> MNITKPFPLPTGYFGIPLGLAALSLAWFHLENLFPAARMVSDVLGIVASAVWILFILMYAYKLRYYFEEVRAEYHSPVRFSFIALIPITTMLVGDILYRWNPLIAEVLIWIGTIGQLLFSTLRVSELWQGGVFEQKSTHPSFYLPAVAANFTSASSLALLGYHDLGYLFFGAGMIAWIIFEPVLLQHLRISSLEPQFRATMGIVLAP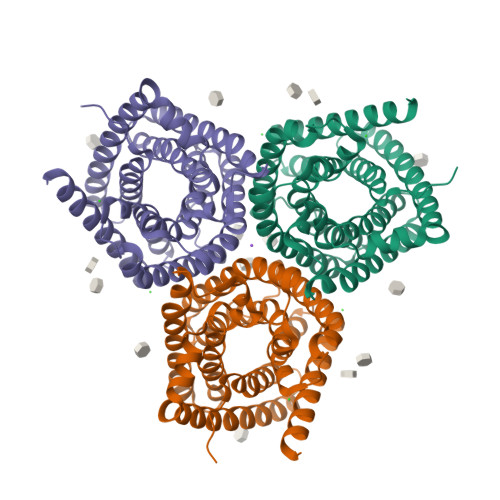AFVCVSAYLSINHGEVDTLAKILWGYGFLQLFFLLRLFPWIVEKGLNIGLWAFSFGLASMANSATAFYHGNVLQGVSIFAFVFSNVMIGLLVLMTIYKLTKGQFFLK> TPVPSTGNPFEGYDIYLSPYYAEEVEAAAAMIDDPVLKAKALKVKEIPTFIWFDVVRKTPDLGRYLADATAIQQRTGRKQLVQIVVYDLPDRDCAAAASNGEFSLADGGMEKYKDYVDRLASEIRKYPDVRIVAVIEPDSLANMVTNMNVAKCRGAEAAYKEGVIYALRQLSALGVYSYVDAGHAGWLGWNA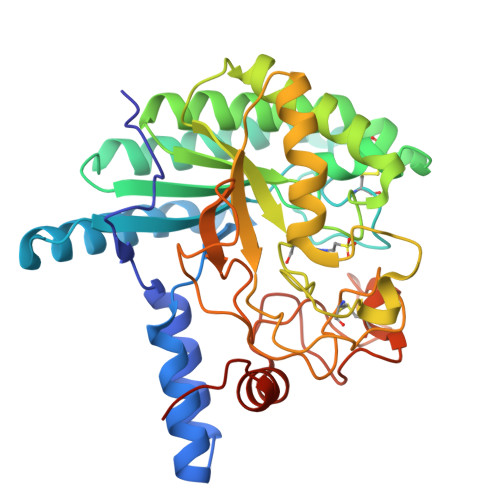NLAPSARLFAQIYKDAGRSAFIRGLATNVSNYNALSATTRDPVTQGNDNYDELRFINALAPLLRNEGWDAKFIVDQGRSGVQNIRQEWGNWCNVYGAGFGMRPTLNTPSSAIDAIVWIKPGGEADGTSDTSAPRYDTHCGKSDSHKPAPEAGTWFQEYFVNLVKNANPPLAAALEHHHHHH>[4x]MKSK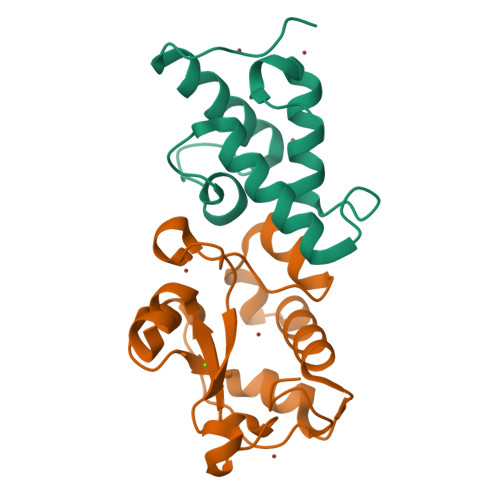ISEYTEKEFLEFVKDIYTNNKKKFPTEESHIQAVLEFKKLTEHPSGSDLLYYPNENREDSPAGVVKEVKEWRASKGLPGFKAGLEHHHHHH;>RDPRDVPGAATGKGQPVSGNWLGAASQGEGAPIPSQIADKLRGKTFKNWRDFREQFWIAVANDPELSKQFNPGSLAVMRDGGAPYVRESEQAGGRIKIEIHHKVRIADGGGVYNMGNLVAVTPKRHIEIHKGGK[4x]>[2x]MSQFDLTPPSPAQRDALIAGLSDEEQRVLLHHGTEAPFCGVFLDNKLDGVYTCRLCGLPLFRSNAKFDSGT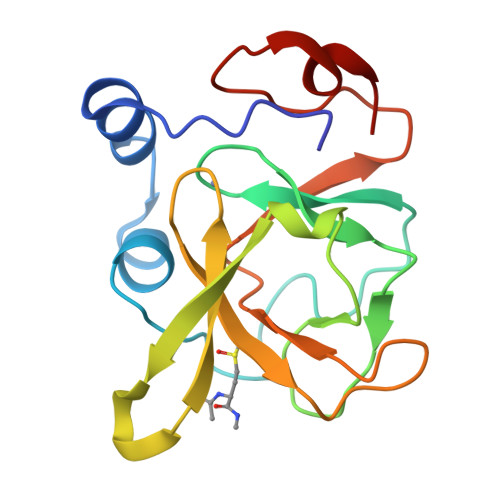GWPSFFAPYDPAHVREIRDTSYGMVRTEIVCARCDSHLGHVFPDGPPPTGERHSLNSVSLAFTEDGQPLPNPLQRAGAETQPA>[2x]GPLGSRPWQILSQALGFPNYDQELWWQNTAETLNRVLEQCDYSVHLQYKYLAFYHKYILPSLGPFRRPGVEPEYISGLSHGGHPLEISVKIDKSKTICRLGLQAIGPLAGTARDPLNSFG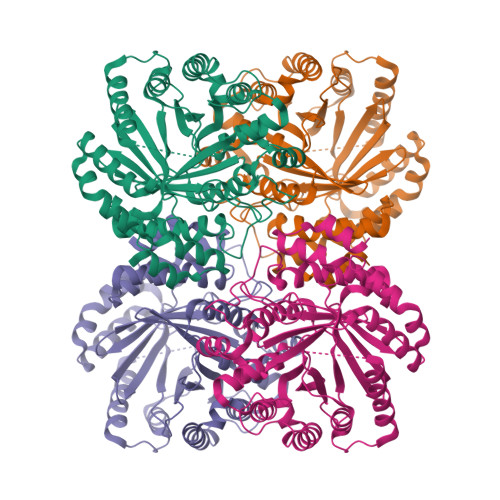DRELLKNLATLLPHVDLRLFDHFNAQVGLDRAQCAVATTKLIKESHNIVCTSLDLKDGEVIPKVYFSTIPKGLVTETPLFDLTFAAIEQMEVYHKDAPLRTALSSLKDFLRPRVPTDASITPPLTGLIGVDCIDPMLSRLKVYLATFRMDLSLIRDYWTLGGLLTDAGTMKGLEMVETLAKTLKLGDEACETLDAERLPFGINYAMKPGTAELAPPQIYFPLLGINDGFIADALVEFFQYMGWEDQANRYKDELKAKFPNVDISQTKNVHRWLGVAYSETKGPSMNIYYDVVAGNVARV> DPCSVTEYSGLATAVSSCKNIVLNGFQVPTGKQLDLSSLQNDSTVTFKGTTTFATTADNDFNPIVISGSNITITGASGHVIDGNGQAYWDGKGSNSNSNQKPDHFIVVQKTTGNSKITNLNIQNWPVHCFDITGSSQLTISGLILDNRAGDKPNAKSGSLP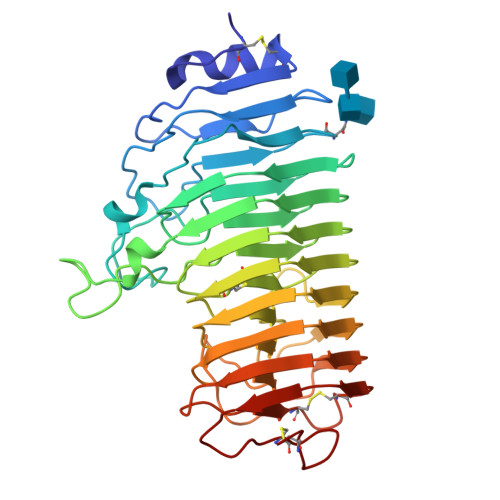AAHNTDGFDISSSDHVTLDNNHVYNQDDCVAVTSGTNIVVSNMYCSGGHGLSIGSVGGKSDNVVDGVQFLSSQVVNSQNGCRIKSNSGATGTINNVTYQNIALTNISTYGVDVQQDYLNGGPTGKPTNGVKISNIKFIKVTGTVASSAQDWFILCGDGSCSGFTFSGNAITGGGKTSSCNYPTNTCPS>[2x]SDWISFSHMSSDTDHFPIKSWFRCEQKAA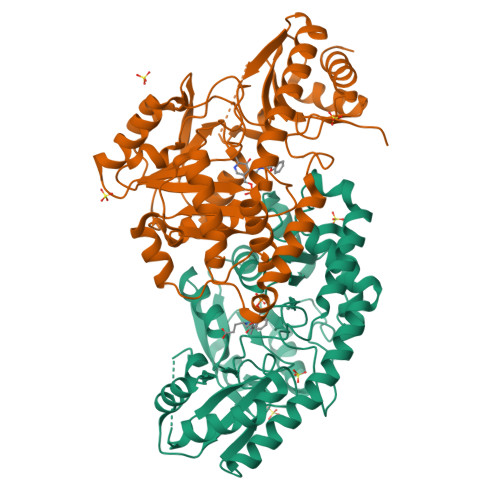SRSYATLGDMSHPQGIYEVRAAITRLISLTRGVKCRPEQMIIGAGTQVLMQLLTELLPKEAVYAMEEPGYRRMYQLLKNAGKQVKTIMLDEKGMSIAEITRQQPDVLVTTPSHQFPSGTIMPVSRRIQLLNWANEEPRRYIIEDDYDSEFTYDVESIPALQSLDRFQNVIYMGTFSKSLLPGLRISYMVLPPELLRAYKQRGYDLQTCSSLTQLTLQEFIESGEYQKHIKKMKQHYKEKRERLITALEAEFSGEVTVKGANAGLHFVTEFDTRRTEQDILSHAAGLQLEIFGMSRFNLKENKRQTGRPTLIIGFARLKEEDIQEGVQRLFKAVYG> MNSAVAGHDQKLNLMQQTMSFLTHDLTQMMPRPVRGDQGQREPALLAGAGV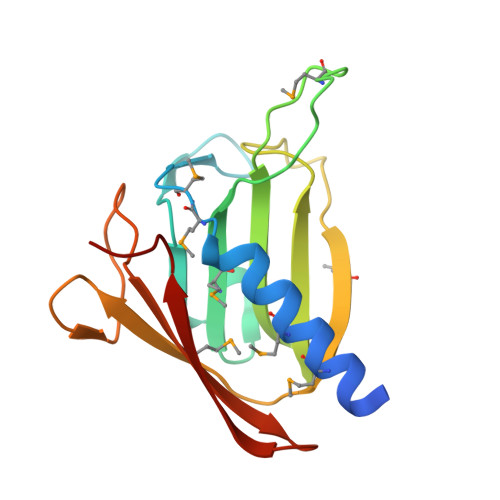LASESEGMRFVRGGVVNPLMRLPRSNLLTVGYRIHDGYLERLAWPLTDAAGSVKPTMQKLIPADSLRLQFYDGTRWQESWSSVQAIPVAVRMTLHSPQWGEIERIWLLRGPQ> GVPTYLLPGSGQFLTTDDHSSAPALPCFNPTPEM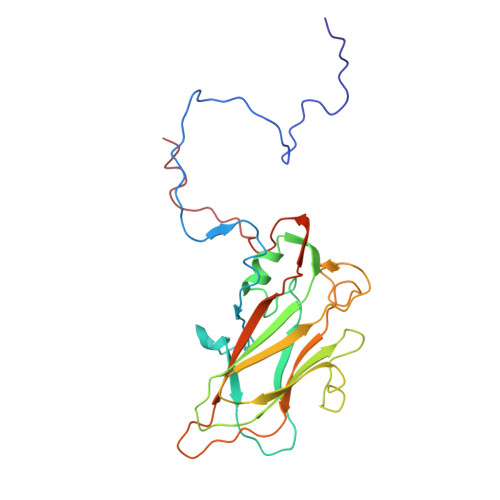HIPGQVRNMLEVVQVESMMEINNTESAVGMERLKVDISALTDVDQLLFNIPLDIQLDGPLRNTLVGNISRYYTHWSGSLEMTFMFCGSFMATGKLILCYTPPGGSCPTTRETAMLGTHIVWDFGLQSSVTLIIPWISGSHYRMFNNDAKSTNANVGYVTCFMQTNLIVPSESSDTCSLIGFIAAKDDFSLRLMRDSPDIGQLDHLHAAEAAYQ> MSGRVGDLSPRQKEALAKFRENVQDVLPALPNPDDYFLLRWLRARSFDLQKSEAMLRKHVEFRKQKDIDNIISWQPPEVIQQYLSGGMCGYDLDGCPVWYDIIGPLDAKGLLFSASKQDLLRTKMRECELLLQECAHQTTKLGRKVETITIIYDCEGLGLKHLWKPAVEAYGEFLCMFEENYPETLKRLFVVKAPKLFPV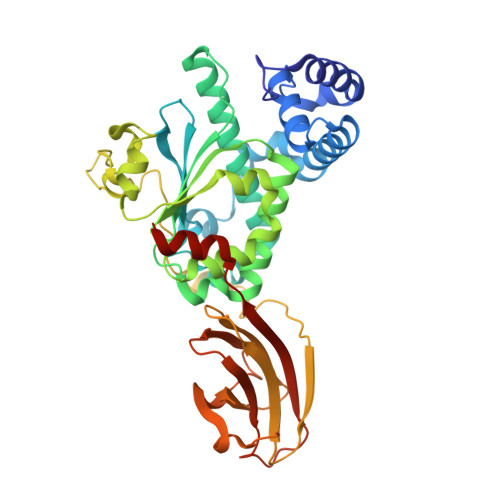AYNLIKPFLSEDTRKKIMVLGANWKEVLLKHISPDQVPVEYGGTMTDPDGNPKCKSKINYGGDIPRKYYVRDQVKQQYEHSVQISRGSSHQVEYEILFPGCVLRWQFMSDGADVGFGIFLKTKMGERQRAGEMTEVLPNQRYNSHLVPEDGTLTCSDPGIYVLRFDNTYSFIHAKKVNFTVEVLLPDKASEEKMKQLGAGTPK>[4x]CGCGA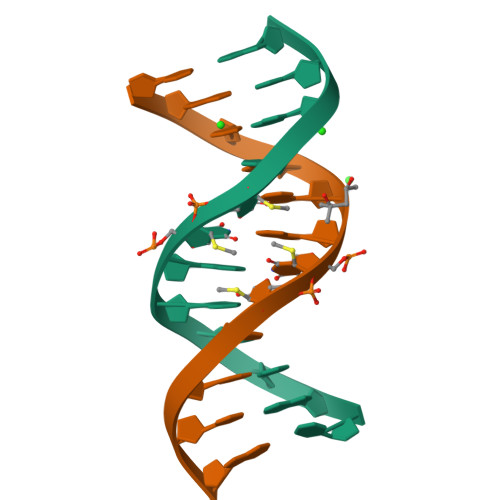AUUCGCG α-Methylacyl-CoA racemase (AMACR; P504S) enzyme plays a vital role in branched-chain fatty acid metabolism by catalyzing the conversion of 2-methyl-branched fatty acyl-CoAs into a near 1 to 1 mixture of the (2R)- and (2S)-epimers, enabling further metabolism. α-Methylacyl-CoA racemase from Mycobacterium tuberculosis (MCR) has been explored as a model to understand the AMACR racemization mechanism and as a drug target. The catalytically active enzyme is a homodimer (with an apparent molecular weight of 83.6 or 89 kDa) with the active site at the interface between the two subunits with catalytic bases contributed by both subunits. Each MCR homodimer contains two active sites formed by residues from the large domain of one subunit and the small domain of the other. Key catalytic residues from the large domain include Asp156 (helix 6) and His126 (helix 5), while Glu241 (beginning of helix 9) is contributed by the small domain.

The 2-methyldecanoyl-CoA 6 side-chain group is a straight-chain group and electron density covered C8, C7, C6 but no density was observed (except in active site H) for the terminal carbons C5, C4, C3, C2, C1 due to conformational heterogeneity (bottom right). Clear electron density for the thioester carbonyl and Cα-Me groups in the ibuprofenoyl-CoA 1 and S-2-methyldecanoyl-CoA 6 complexes shows a cis conformation. The thioester oxygen forms hydrogen bonds with Asp127, Asp156, and His126. In 2-methylacyl-CoA structures, Fo–Fc maps did not favor R- or S-epimers; both were refined with full occupancy. The Cα-H of each epimer points toward His126 or Asp156, resulting in distinct rotations around the Cα atom. Ibuprofenoyl-CoA 1 and analogs and 2-methyldecanoyl-CoA 6 were relatively potent inhibitors, with ibuprofenoyl-CoA 1 displaying the highest levels of potency (pIC50 = 5.05 ± 0.05; mean ± SEM, n = 3). Our results are consistent with a different mechanism in which the side-chain is held in a relatively static position with the different stereochemical configurations accommodated by a subtle clockwise or anticlockwise rotation of the α-carbon. The crystal structures for ibuprofenoyl-CoA 1, other 2-APA-CoA substrates 2-5, and 2-methyldecanoyl-CoA 6 demonstrate that this mechanism applies to all these substrates. We therefore performed a similar analysis for ibuprofenoyl-CoA 1 and analogs, and 2-methyldecanoyl-CoA 6. This analysis showed that potency was negatively correlated with LogP for these compounds, that is potency was decreased with increasing LogP values.

>[12x]MAGPLSGLRVVELAGIGPGPHAAMILGDLGADVVRIDRPSSVDGISRDAMLRNRRIVTADLKSDQGLELALKLIAKADVLIEGYRPGVTERLGLGPEECAKVNDRLIYARMTGWGQTGPRSQQAGHDINYISLNGILHAIGRGDERPVPPLNLVGDFGGGSMFLLVGILAALWERQSSGKGQVVDAAMVDGSSVLIQMMWAMRATGMWTDTRGANMLDGGAPYYDTYECADGRYVAVGAIEPQFYAAMLAGLGLDAAELPPQNDRARWPELRALLTEAFASHDRDHWGAVFANSDACVTPVLAFGEVHNEPHIIERNTFYEANGGWQPMPAPRFSRTASSQPRPPAATIDIEAVLTDWDGGSGC> TLMTGQ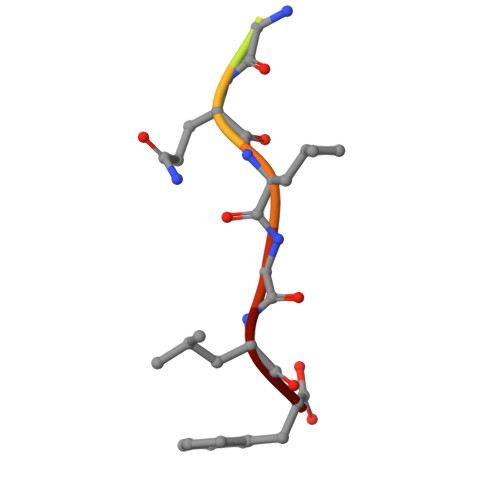LGLF> SSTMGQVGRQLAIIGDDINRRYG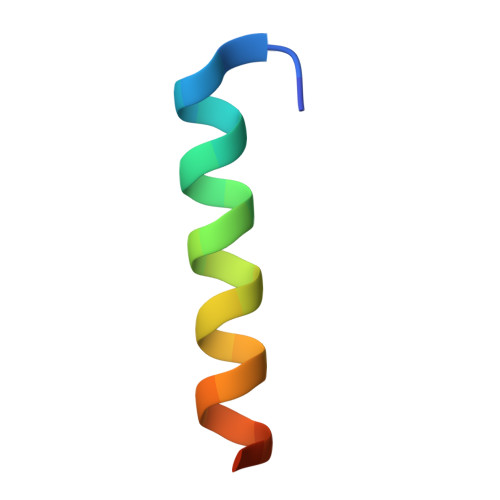GC> MASPIESARIGEVKRETKETNVSVKINLDGHGVSDSSTGIPFLDHMLDQLASHGLFDVHVRATGDTHIDDHHTNEDVALAIGTALLKALGERKGINRFGDFTAPLDEALIHVSLDLSGRPYLGYNLEIPTQRVGTYDTQLVEHFFQSLVNTSGMTLHIRQLAGKNSHHIIEATFKAFARALRQATESDPRRGGTIPSSKGVLSRS

The program of herbicide development described herein aims to identify inhibitors of imidazoleglycerolphosphate‐dehydratase (IGPD; EC 4.2.1.19), an enzyme of histidine biosynthesis in plants and microorganisms. This enzyme catalyzes the manganese(II)‐dependent dehydration of (2R,3S)‐2,3‐dihydroxy‐3‐(1H‐imidazol‐5‐yl)propyl dihydrogen phosphate (2R,3S‐IGP) to 3‐(1H‐Imidazol‐4‐yl)‐2‐oxopropyl dihydrogen phosphate (IAP).4 IGPD shows strict enantioselectivity for its substrate, with the other three diastereoisomers of IGP acting as competitive inhibitors of the enzyme, thus indicating that the active site shows some flexibility to accommodate inverted chiral centers. Previous studies have shown that IGPD is inhibited by triazolylphosphonates, whose potency is based on mimicking key reaction intermediates. In this paper we describe work on the lead compound, 2‐hydroxy‐3‐(1,2,4‐triazol‐1‐yl) propylphosphonate (C348) and present a series of structures of IGPD, from Arabidopsis thaliana, complexed with a synthetic racemate of C348 and with the enantiopure compounds.

In this study, weak electron density was observed adjacent to the chiral center of the lead compound in a 1.85 Å resolution structure of our target enzyme in complex with a racemate. However, as with the electron density for C348 in the 1.85 Å structure, the density at 1.1 Å resolution was also weak around C3. Nevertheless, a small peak could be observed in the map around C3 when contoured at 1 σ, the position of which was consistent with the binding of the (S)‐C348. Refinement of this structure using tight geometric restraints revealed further difference features, indicating a second position for the inhibitor, which, from the geometry, could only be interpreted as resulting from the binding of the (R)‐C348. This finding indicated that in the crystal, the active sites of some of the enzyme molecules were occupied by (S)‐C348 and others were occupied by (R)‐C348. Subsequent refinement of this structure with occupancies of 0.6 and 0.4 for the (S)‐ and (R)‐C348, respectively, produced a model which fully explained the electron density, thus indicating that both enantiomers of C348 were bound to an essentially invariant enzyme structure. The two enantiomers thus trace an inverted path between the metal binding site and the phosphonate binding site, whereby they are related by mirror‐image packing. Both enantiomers retain low‐energy conformations with approximately staggered torsion angles, with the largest deviation in the atomic position of equivalent atoms occurring at C3 of the backbone, thus explaining the weak density at this position observed in the complexes of IGPD2 with the racemate. By extending the resolution and chirally resolving the two enantiomers we confirmed that the areas of weakness arose from the mirror‐image packing of the two enantiomers of the inhibitor in the active site, an observation not without precedence.> RRASRFAQWAIHPTFNLKSLSCSLEVSKDSRTVTVSHRPQPYRWSCERFSTSQVLCSQALSSGKHYWEVDTRNCSHWAVGVASWEMSRDQVLGRTMDSCCVEWKGTSQLSAWHMVKETVLGSDRPGVVGIWLNLEEGKLAFYSVDNQEKLLYECTISASSPLYPAFWLYGLH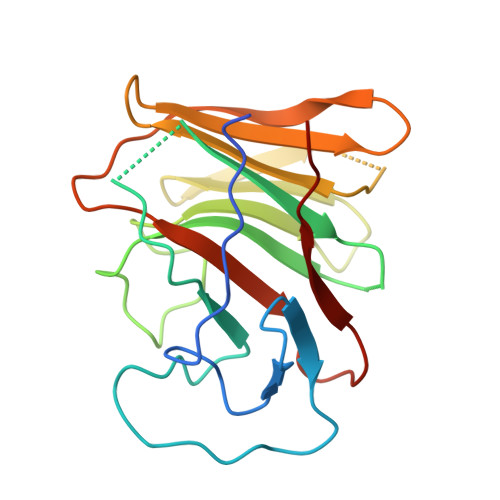PGNYLIIKQVKV>[4x]SKSRRWVFALRHGERVDLTYGPWVPHCFENDTYVRKDLNLPLKLAHRAGGKGGYVKDTPLTRLGWFQAQLVGEGMRMAGVSIKHVYASPALRCVETAQGFLDGLRADPSVKIKVEPGLFEFKNWHMPKGIDFMTPIELCKAGLNVDMTYKPYVEMDASAETMDEFFKRGEVAMQAAVNDTEKDGGNVIFIGHAITLDQMVGALH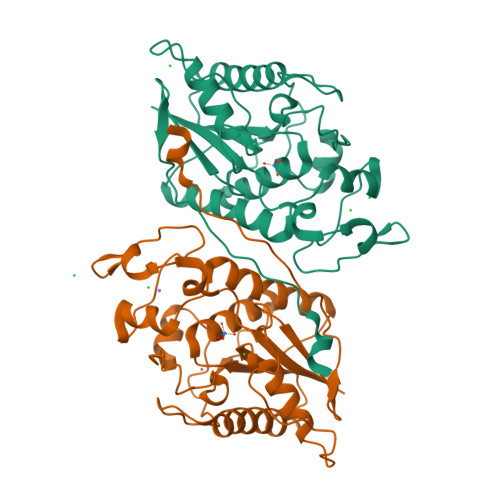RLRDDMEDVQPYEIGRNLLKVPYCALGAMRGKPWDVVSPPCPPSINSSSGRFDWRILIK> SN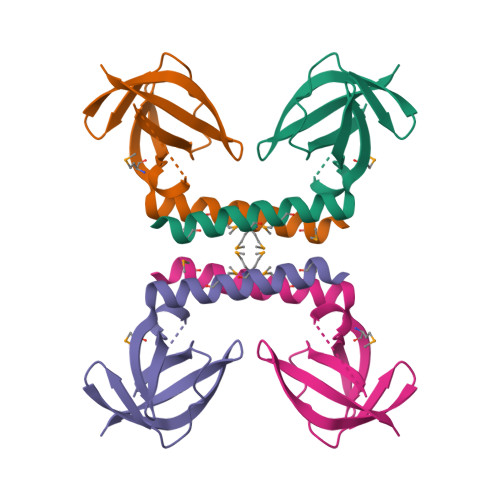AMADLFDGMKRRMDALIAERFGMKVNINGTDCIVVESDFLAELGPVEGNGKNVVVFSGNVIPRRGDRVVLRGSEFTVTRIRRFNGKPQLTLEENNGGKGA> GAMGPLEEAIKDVDVSGVLRYRYDTGNFDKNFLNNSNLNNSKQDHKYRAQVNFSAAIADNFKAFVQFDYNAVDGGTGVDNATNAEKGLFVRQLYLTYTNEDVATSVIAGKQQLNIIWTDNGVDGLVGTGVKVVNNSIDGLTLAAFAVDSFMAAEQGSDLLGQSTYVGNGKNNNDSFKLDSIGNLYGAAAVGSYDLAGGQFNPQLWLAYWDQVAFFYAVDAAYSTTIFDGINWTLEGAYLGNSLDSELDDKKTYANGNLFALKGSIEVNGWDASLGGLYYGDKEKASTVVIEDQGNLGSLLAGEEIFYTTGSRLNGDTGRNIFGYVTGGYTFNETVRVGADFVYGGTKTEATTHLGGGKKLEAVARVDYKYSPKLNFSAFYSYVNLDQGVNTNESADHSTVRLQALYKF

In contrast to E. coli, C. jejuni has only one major outer membrane protein (MOMP), which is thus far present in all isolates and is highly (but not absolutely) conserved in other Campylobacteria. MOMP is an 18-stranded antiparallel β-barrel porin with an elliptical shape common to other 18-stranded porins. Unusually for an 18-stranded β-barrel, MOMP adopts the same trimeric arrangement as seen for OmpF and OmpC, which are 16-stranded β-barrels. The most striking difference between MOMP and OmpF/OmpC from E. coli is the presence of a Ca2 +-binding site in the constriction zone of MOMP.

The structure of the overexpressed selenomethionine (SeMet) variant MOMP was solved using single-wavelength anomalous diffraction to provide initial phases, which were improved by density modification. This structure was then used to solve the high-resolution structure of MOMP purified from an E. coli overexpression system (rMOMP). Our discussion focuses on the higher-resolution rMOMP structure (2.1 Å). In rMOMP, however, due to cloning artifacts, we have three additional non-native residues after signal peptide cleavage (Gly-Ala-Met), followed by a single point mutation of Thr1 to Gly. We observed additional electron density adjacent to L3 and L4 that we identify as a Ca2 + (rather than Zn2 + or Mg2+, or K+ or Na+) based on electron density and coordination (distance and geometry). The proteins expressed in E. coli have not had any Ca2 + ion added and we conclude that the ion was bound during expression in E. coli and has remained attached in throughput purification. The ion has octahedral coordination, with one oxygen atom from the side chain of Asp120, Gln152, Asp155, and Glu288, and has the carbonyl of Asp120 with a water molecule filling the final sixth position. The metal ion creates a cross-link among L3, L4, and L6. Additionally, the difference electron density map showed a residual elongated density that was modeled as an ethylene glycol like the molecule [from polyethylene glycol (PEG) 400 or C8E4] in the rMOMP. This molecule sits below the constriction zone underneath L3. Although only one monomer is present in the asymmetric unit, analysis of the crystal packing reveals a trimeric arrangement reminiscent of that seen in OmpC and OmpF.>[8x]MLWKKSLSELRELLKRGEVSPKEVVESFYDRYNQTEEKVKAYITPLYGKALKQAESLKERELPLFGIPIAVKDNILVEGEKTTCASKILENFVAPYDATVIERLKKAGALIVGKTNLDEFAMGSSTEYSAFFPTKNPWDLERVPGGSSGGSAASVAVLSAPVSLGSDTGGSIRQPASFCGVIGIKPTYGRVSRYGLVAFASSLDQIGVFGRRTEDVALVLEVI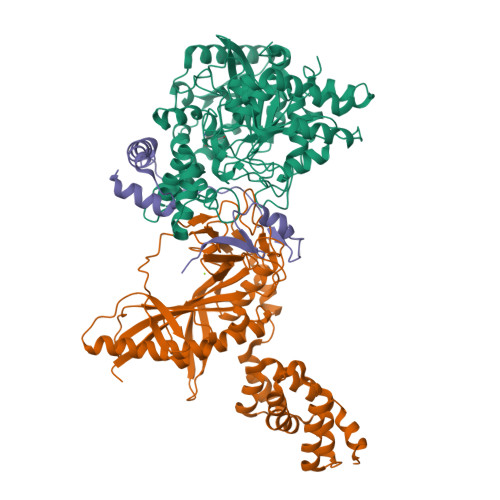SGWDEKDSTSAKVPVPEWSEEVKKEVKGLKIGLPKEFFEYELQPQVKEAFENFIKELEKEGFEIKEVSLPHVKYSIPTYYIIAPSEASSNLARYDGVRYGYRAKEYKDIFEMYARTRDEGFGPEVKRRIMLGTFALSAGYYDAYYLKAQKVRRLITNDFLKAFEEVDVIASPTTPTLPFKFGERLENPIEMYLSDILTVPANLAGLPAISIPIAWKDGLPVGGQLIGKHWDETTLLQISYLWEQKFKHYEKIPLT;>[8x]MNEKYEAVIGLEIHVQMDTKTKMFCGCKVEFGAEPNTNVCPVCLGMPGALPIVNKRAVEYAIRASLALNCEVHEESVFARKHYFYPDLPKGYQISQYEKPLATNGWVELNLPNGEKKKVRIRRLHIEEDAGKNIHEGDKTLVDLNRAGTPLMEIVTEPDIRTPEEARLFLEKLRNIMRYAGVSKADMEKGQLRCDINVSIRPKGSKEFGTRVEIKNVNSFRFVQKALEYEIERQINVVEEGGEVVQETRTFDPQTGKTYPMRTKEEAEDYRYFPDPDLVPLKVKKEWIEEIKKNMPELPDQRFERLIKEYGLSEYEAGILVNHKEVGDFFEEAVRHFKEPKGIVNWLINDLLGLLRDKGISIEESPVKPEHLAELVKLIKEKVISTKIGKEVIKEMVETGKTPSQIVEEKGLKQITDENQIKELVKKIFEKHPKEVERLKQGEEKLIGFFVGQVMRETRGKANPQVVNKVIRELVKEV;>MVDREWVLKIAKLARLELKEEEIEVFQKQLSDILDFIDQLKELDTENVEPYIQEFEETPMREDEPHPSLDREKALMNAPERKDGFFVVPRVVEV[8x]> ANPLYQKHIISINDLSRDDLNLVLATAAKLKANPQPELLKHKVIASCFFEASTRTRLSFETSMHRLGASVVGFSDSANTSLGKKGETLADTISVISTYVDAIVMRHPQEGAARLATEFSGNVPVLNAGDGSNQHPTATLLDLFTIQETQGRLDNLHVAMVGDLKYGRTVHSLTQALAKFDGNRFYFIAPDALAMPQYILDMLDEKGIAWSLHSSIEEVMAEVDILYMTRVQKERLDPSEYANVKAQFVLRASDLHNAKANMKVLHPLPRVDEIATD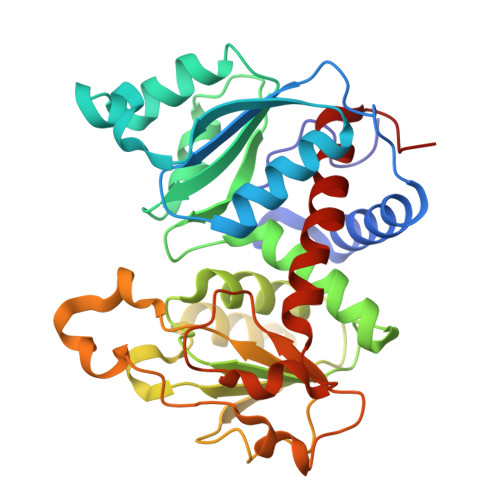VDKTPHAWYFQQAGNGIFARQALLALVLNRDLVL> MSQAIGILELTSIAKGMELGDAMLKSANVDLLVSKTISPGKFLLMLGGDIGAIQQAIETGTSQAGEMLVDSLVLANIHPSVLPAISGLNSVDKRQAVGIVETWSVA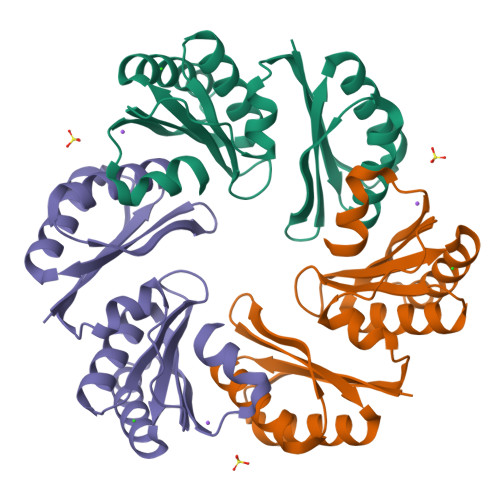ACISAADRAVKGSNVTLVRVHMAFGIGGKCYMVVAGDVSDVNNAVTVASESAGEKGLLVYRSVIPRPHEAMWRQMVEGLEHHHHHH> M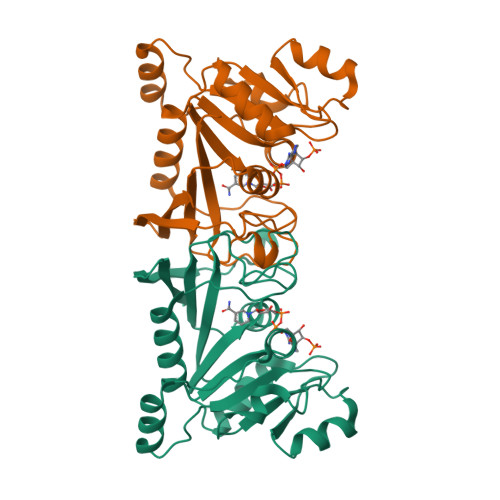RGSHHHHHHGSMDRPFIFINSAMSADGKLSTKERKQVKISGKLAFERMDELRAHADAIMVGIGTVLADDPSLTVKSPERKAARKAAGKSENPVRVVVDSSARTPLNADIFKKGEGLRIIAVSNSAPEEKIRMLEEKALVIKTGAFRVDLTELAAKLKEMGINSLMVEGGATLNWGMLSAGLVDEVYTFVGNLIIGGKTAPTFTDGEGFTENELLGLELSSAEKIEDGILLKWKVKGKKN> PKQKAQLDELSMSEKIAILLIQVGEDTTGEILRHLDIDSITEISKQIVQLNGTDKQIGAAVLEEFFAIFQSNQY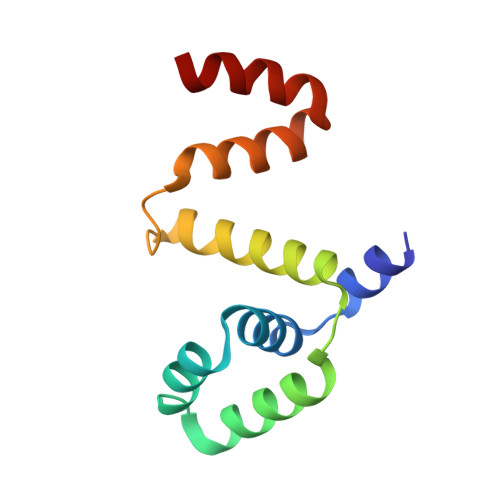INTGGLEYARELLTRTLGSEEAKKVMDKLTK> 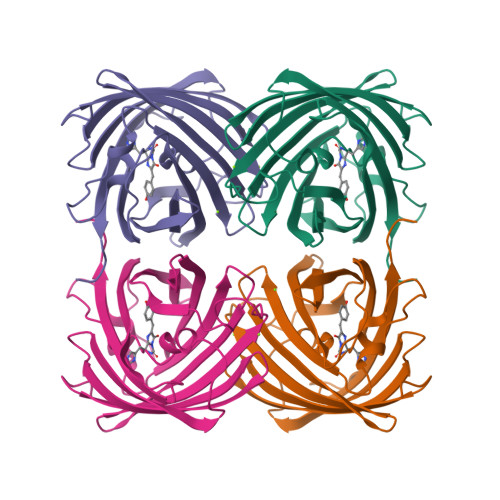MSVIKSDMKIKLRMEGTVNGHKFVIEGEGEGKPYEGTQTMNLKVKEGAPLPFAYDILTTVFHYGNRVFAKYPKHIPDYFKQSFPEGYSWERSMTFEDGGICTARNDITLEGDCFFYEIRFDGVNFPPNGPVMQKKTLKWEPSTEKMYVRDGVLTGDINMALLLEGGGHYRCDFKTTYKAKKGVQLPDYHFVDHCIEILSHDKDYNNVKLYEHAVAHSGLPRQAKHHHHHH>[2x]AGFQLNEFSSSGLGRAYSGEGAIADDAGNVSRNPALITMFDRPTFSAGAVYIDPDVNISGTSPS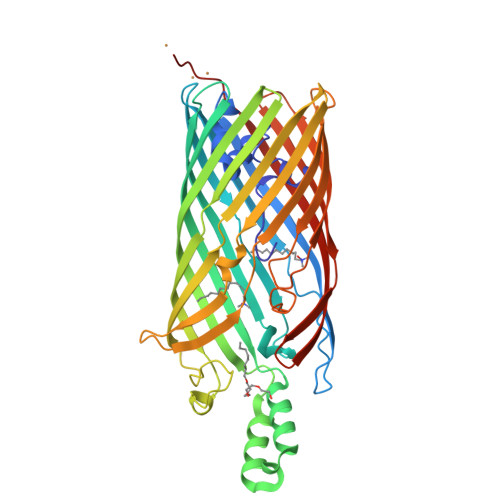GRSLKADNIAPTAWVPNMHFVAPINDQFGWGASITSNYGLATEFNDTYAGGSVGGTTDLETMNLNLSGAYRLNNAWSFGLGFNAVYARAKIERFAGDLGQLVAGQIMQSPAGQTQQGQALAATANGIDSNTKIAHLNGNQWGFGWNAGILYELDKNNRYALTYRSEVKIDFKGNYSSDLNRAFNNYGLPIPTATGGATQSGYLTLNLPEMWEVSGYNRVDPQWAIHYSLAYTSWSQFQQLKATSTSGDTLFQKHEGFKDAYRIALGTTYYYDDNWTFRTGIAFDDSPVPAQNRSISIPDQDRFWLSAGTTYAFNKDASVDVGVSYMHGQSVKINEGPYQFESEGKAWLFGTNFNYAFHHHHHH>[2x]KKKIVDANIATETMIDINVGGAIFETSRHTLTQQKDSFIEKLLSGRHHVTRDKQGRIFLDRDSELFRIILNFLRNPLTIPIPKDLSESEALLKEAEFYGIKFLPFPLVFCIGGFDGVEYLNSMELLDISQQCWRMCTPMSTKKAYFGSAVLNNFL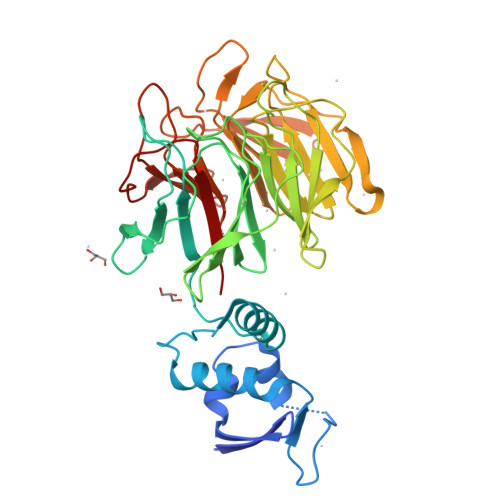YVFGGNNYDYKALFETEVYDRLRDVWYVSSNLNIPRRNNCGVTSNGRIYCIGGYDGSSIIPNVEAYDHRMKAWVEVAPLNTPRSSAMCVAFDNKIYVIGGTNGERLNSIEVYEEKMNKWEQFPYALLEARSSGAAFNYLNQIYVVGGIDNEHNILDSVEQYQPFNKRWQFLNGVPEKKMNFGAATLSDSYIITGGENGEVLNSCHFFSPDTNEWQLGPSLLVPRFGHSVLIANI>SLFELGKMILQETGKNPAKSYGAYGCNCGVLGRGQPKDATDRCCYVHKCCYKKLTGCDPKKDRYSYSWKDKTIVCGENNPCLKELCECDKAVAICLRENLGTYNKKYRYHLKPFCKKADPC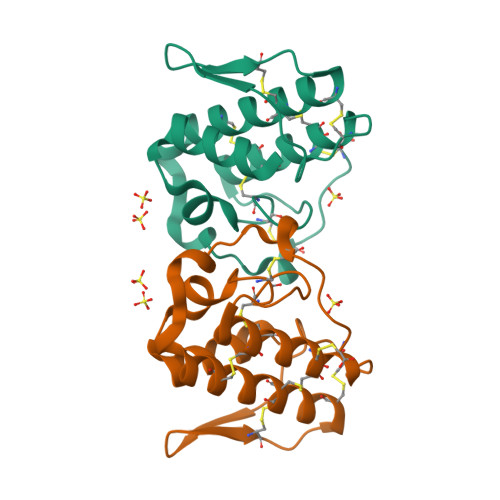[2x]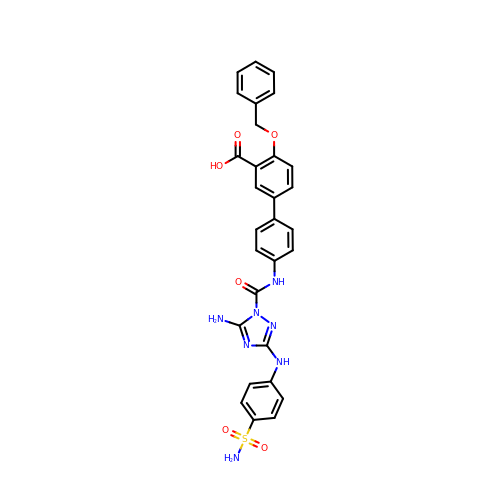4'-{[5-amino-3-(4-sulfamoylanilino)-1H-1,2,4-triazole-1-carbonyl]amino}-4-(benzyloxy)[1,1'-biphenyl]-3-carboxylic acid | C29 H25 N7 O6 S | KMNBCUUTUMNJGS-UHFFFAOYSA-N> MSGTRASNDRPPGTGGVKRGRLQQEAAATGSRVTVVLGAQWGDEGKGKVVDLLATDADIVSRCQGGNNAGHTVVVDGKEYDFHLLPSGIINTKAVSFIGNGVVIHLPGLFEEAEKNEKKGLKDWEKRLIISDRAHLVFDFHQAVDGLQEVQRQAQEGKNIGTTKKGIGPTYSSKAARTGLRICDLLSDFDEFSARF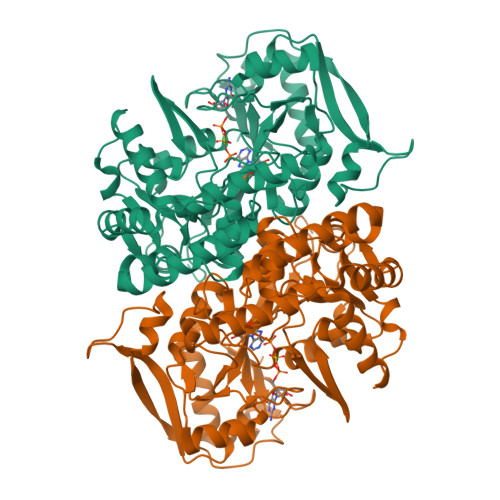KNLAHQHQSMFPTLEIDVEGQLKRLKGFAERIRPMVRDGVYFMYEALHGPPKKVLVEGANAALLDIDFGTYPFVTSSNCTVGGVCTGLGIPPQNIGDVYGVVKAYTTRVGIGAFPTEQINEIGDLLQNRGHEWGVTTGRKRRCGWLDLMILRYAHMVNGFTALALTKLDILDVLSEIKVGISYKLNGKRIPYFPANQEILQKVEVEYETLPGWKADTTGARKWEDLPPQAQSYVRFVENHMGVAVKWVGVGKSRESMIQLF>[2x]GSMTNRTDDEYPEAPSDRTHVKRYHWLARYDQETVKAILDATPLAHVGCMMNGVPFVTPTFFWREGDRVYWHGSSAGRLFKALEHQDICLTVSLLDGLVIARSAYNFNCNFRSVMLLGRAELISDEAVKAEKLRNFVDGLIPGEWERLRPVHAKEIEATAVASLSIAEASCKVRTGPPLDDEEDYAFPSWAGVIPIRYQVLPPEPDPRNLPDVPMPEDILKFRLG

Here, we have structurally and functionally characterized Anf3 from A. vinelandii and identified it as a flavocytochrome. The protein is a dimer and homologous to flavin-binding domains of the pyridoxamine 5′-phosphate oxidase family. Anf3 is a terminal oxygen oxidoreductase with ferredoxin or flavodoxin as the probable physiological electron donor. The terminal oxidase activity of the protein suggests an oxygen scavenging function to protect the iron-only nitrogenase.

Anf3 was overexpressed in Escherichia coli, aerobically purified, and crystallized, and the structure determined to atomic resolution. The asymmetric unit contained a dimer, the subunits are in similar conformations with a Cα RMSD6 of 0.2 Å. Each monomer core is a split-barrel flavin-binding domain that binds an FAD and also a b-type heme. Two loops from residues 96–107 and 172 to the C terminus leave the core, interact with the other monomer, and loop back. The dimer is tightly intertwined, and the cofactors interact with both monomers. The heme iron is ligated by a proximal histidine, His70, and an axial water molecule. Two conserved residues, Arg21 and Lys170 hydrogen-bond the heme propionates, stabilizing the heme–protein complex and controlling heme poise. The heme porphyrin ring is 3.4 Å from the isoalloxazine ring of the FAD at the closest point, consistent with a π-stacking interaction. At the entrance to the active site there is a tyrosine (Tyr22) that is hydrogen-bonded to a water molecule that forms part of a chain of two water molecules hydrogen-bonded to the heme axial water. This network is a candidate for a proton relay, necessary for rapid delivery of protons to the substrate oxygen when it is reduced.> MHHHHHHMELSLA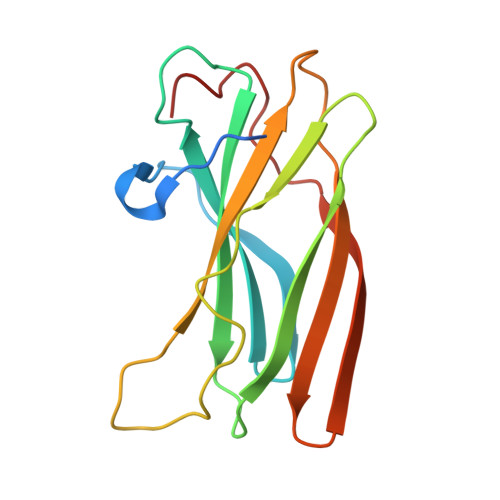SITVPLESIKPSNILPVTVYDQHGFRILFHFARDPLPGRSDVLVVVVSMLSTAPQPIRNIVFQSAVPKVMKVKLQPPSGTELPAFNPIVHPSAITQVLLLANPQKEKVRLRYKLTFTMGDQTYNEMGDVDQFPPPETWGSL>GSHMPDPDDGLTFRVLSMHDVRDNLRASFADMPDQFAIETRTLTDLFEWIRVKGFNPISMQQIIDSRAGVRPLPPRPILLTFDDGYASTYTKVFPLLAAFNYPAVVAVVTSWTDAPAGTKIRLSPKIEVPHDFFMTWAQLREMAQSGLVELASHSHNLHRGVLANPQGNEQPAASSRQYLPASGRYENDAEYRARVRQDLKTSAHLIRHHTGVTIRSIVWPYGAHNRDTDQVAAEVGLNIGLTLQPGPNTPDVALTQIRRSLVDYEVNVATV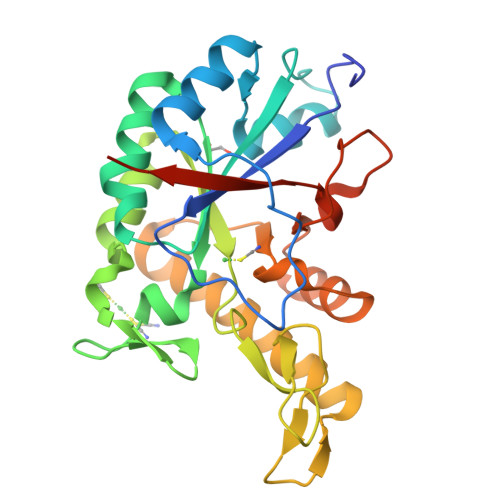ARAMR[2x]> GPMLGKHWSEKKLEEMKERDWRIFKENFGISTKGGSIPNPMRNWEESGLPRRLLDIVYRVGYDEPTPIQRAAIPIALQARDLIGVAVTGSGKTAAFLLPLLVYISELPPLTEYNKNDGPYALILAPTRELVQQIE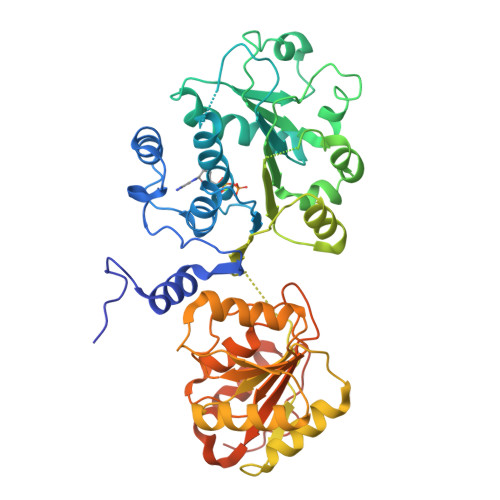SEARKFADPLGFTVVSIVGGHSLEEQAFALRNGAEIIVATPGRLVDCIERRLLVFSQCCYVIMDEADRMIDQGFEEPLTKILDALPVSNEKPDTEDAENPQLMSRYLGGRDRYRQTMMYTATMPPTVEKIAKKYLRRPAIVTIGNAGEAVDTVEQRVEFIAGEDKRKRRLQEILNSGQFKPPIIVFVNIKRNCEMVAKDIKSWGFSTVTLHGSKTQEQREASLAALRNGQAHILVATDLAGRGIDVPDVSLVVNFNMPSTIEAYTHRIGRTGRAGKSGVAITFLGNEDADVMYDLKQIISKSSISKVPEELRRHEAAQSKPNRVKKIEDSSGFAGKGGWQ>MLVKGNEILLKAHKEGYGVGAFNFVNFEMLNAIFEAGNEENSPLFIQASEGAIKYMGIDMAVGMVKIMCERYPHIPVALHLDHGTTFESCEKAVKAGFTSVMIDASHHAFEENLELTSKVVKMAHNAGVSVEAELGRLMGIEDNISVDAKDAVLVNPKEAEQFVKESQVDYLAPAIGTSHGAFKFKGEPKLDFERLQEVKRLTNIPLVLHGASAIPDNVRKSYLDAGGDLKGSKGVPFEFLQESVKGGINKVNTDTDLR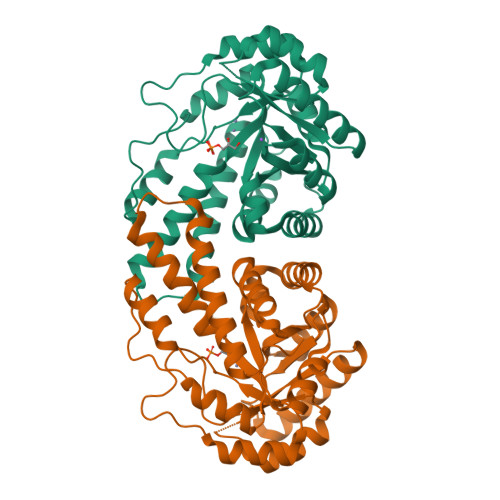IAFIAEVRKVANEDKSQFDLRKFFSPAQLALKNVVKERMKLLGSANKI[2x]N-(tert-butoxycarbonyl)-L-tyrosine | C14 H19 N O5 | 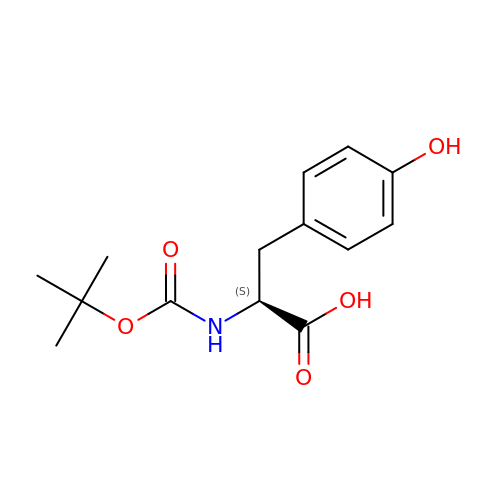CNBUSIJNWNXLQQ-NSHDSACASA-N>[2x]MLTGLNHLTLAVADLPASIA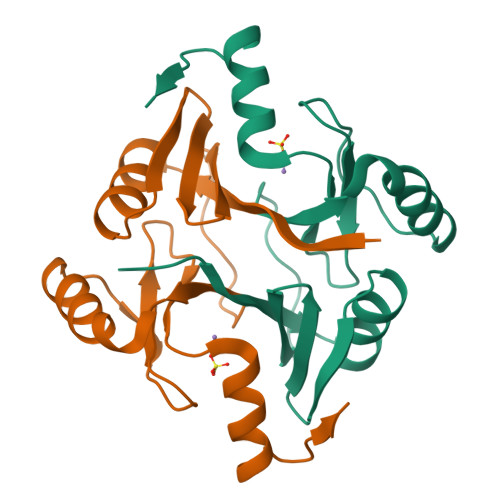FYRDLLGFRLEARWDQGAYLELGSLWLCLSREPQYGGPAADYTHYAFGIAAADFARFAAQLRAHGVREWKQNRSEGDSFYFLDPDGHRLEAHVGDLRSRLAACRQAPYAGMRFAD> GPHMSSERVLSYAPAFKSFLDTSFFQELSRLKLDVLKLDSTCQPLTVNLDLHNIPKSADQVPLFLTNRSFEKHNNKRTNEVPLQGSIFNFNVLDEFKNLDKQLFLHQRALECWEDGIKDINKCVSFVIISFADLKKYRFYY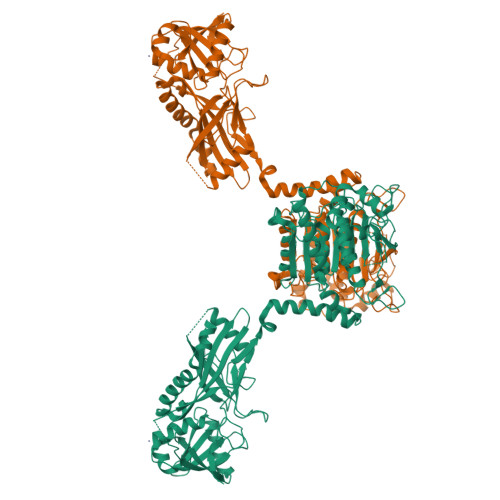WLGVPCFQRPSSTVLHVRPEPSLKGLFSKCQKWFDVNYSKWVCILDADDEIVNYDKCIIRKTKVLAIRDTSTMENVPSALTKNFLSVLQYDVPDLIDFKLLIIRQNEGSFALNATFASIDPQSSSSNPDMKVSGWERNVQGKLAPRVVDLSSLLDPLKIADQSVDLNLKLMKWRILPDLNLDIIKNTKVLLLGAGTLGCYVSRALIAWGVRKITFVDNGTVSYSNPVRQALYNFEDCGKPKAELAAASLKRIFPLMDATGVKLSIPMIGHKLVNEEAQHKDFDRLRALIKEHDIIFLLVDSRESRWLPSLLSNIENKTVINAALGFDSYLVMRHGNRDEQSSKQLGCYFCHDVVAPTDSLTDRTLDQMCTVTRPGVAMMASSLAVELMTSLLQTKYSGSETTVLGDIPHQIRGFLHNFSILKLETPAYEHCPACSPKVIEAFTDLGWEFVKKALEHPLYLEEISGLSVIKQEVER>[2x]HMTDGERQNATEIRASVGKMIDGIGRFYIQMCTELKLSDYEGRLI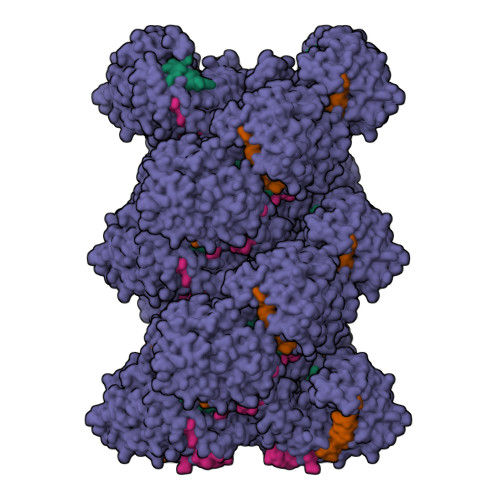QNSLTIERMVLSAFDERRNKYLEEHPSAGKDPKKTGGPIYRRVDGKWRRELILYDKEEIRRIWRQANNGDDATAGLTHMMIWHSNLNDATYQRTRALVRTGMDPRMCSLMQGSTLPRRSGAAGAAVKGVGTMVMELIRMIKRGINDRNFWRGENGRRTRIAYERMCNILKGKFQTAAQRTMVDQVRESRNPGNAEFEDLIFLARSALILRGSVAHKSCLPACVYGSAVASGYDFEREGYSLVGIDPFRLLQNSQVYSLIRPNENPAHKSQLVWMACHSAAFEDLRVSSFIRGTKVVPRGKLSTRGVQIASNENMETMESSTLELRSRYWAIRTRSGGNTNQQRASSGQISIQPTFSVQRNLPFDRPTIMAAFTGNTEGRTSDMRTEIIRLMESARPEDVSFQGRGVFELSDEKATSPIVPSFDMSNEGSYFFGDNAEEYDNLEHHHHHH> GSVGNREEKILNREIGFAIGMPVCEFDMVKDPEVQDFRRNILNVCKEAVDLRDLNSPHSRAMYVYPPNVESSPELPKHIYNKLDKGQIIVVIWVIVSPNNDKQKYTLKINHDCVPEQVIAEAIRKKTRSMLLSSEQLKLCVLEYQGKYILKVCGCDEYFLEKYPLSQYKYIRSCIMLGRMPNLMLMAKESLYSQLPMDCFTMPSYSRRISTATPYMNGETSTKSLWVINSALRIKILCATYVNVNIRDIDKIYVRTGIYHGGEPLCDNVNTQRVPCSNPRWNEWLNYDIYIPDLPRAARLCLSICSVKGRKGAKEEHCPLAWGNINLFDYTDTLVSGKMALNLWPVPHGLEDLLNPIGVTGSNPNKETPCLELEFDWFSSVVKFPDMSVIEEHANWSVSREAGFSYSHAGLSNRLARDNELRENDKEQLKAISTRDPLSEITEQEKDFLWSHRHYCVTIPEILPKLLLSVKWNSRDEVAQMYCLVKDWPPIKPEQAMELLDCNYPDPMVRGFAVRCLEKYLTDDKLSQYLIQLVQVLKYEQYLDNLLVRFLLKKALTNQRIGHFFFWHLKSEMHNKTVSQRFGLLLESYCRACGMYLKHLNRQVEAMEKLINLTDILKQEKKDETQKVQMKFLVEQMRRPDFMDALQGFLSPLNPAHQLGNLRLEECRIMSSAKRPLWLNWENPDIMSELLFQNNEIIFKNGDDLRQDMLTLQIIRIMENIWQNQGLDLRMLPYGCLSIGDCVGLIEVVRNSHTIMQIQCKGGLKGALQFNSHTLHQWLKDKNKGEIYDAAIDLFTRSCAGYCVATFILGIGDRHNSNIMVKDDGQLFHIDFGHFLDHKKKKFGYKRERVPFVLTQDFLIVISKGAQECTKTREFERFQEMCYKAYLAIRQHANLFINLFSMMLGSGMPELQSFDDIAYIRKTLALDKTEQEALEYFMKQMNDAHH

Class IA PI3Ks signal downstream of tyrosine kinases, G protein-coupled receptors and small GTPases to regulate cell metabolism, growth, proliferation and migration. They consist of a p110α, β or δ catalytic subunit and a p85 regulatory subunit (further referred to as PI3Kα, PI3Kβ and PI3Kδ), with a broad tissue distribution (p110α, p110β) or enriched in leukocytes (p110δ). PI3Kα phosphorylates PIP2 in the plasma membrane to PtdIns(3,4,5)P3 (or PIP3), which can be converted by 5-phosphatases to PtdIns(3,4)P2. Here we report on the discovery of UCL-TRO-1938 (further referred to as 1938), a small molecule activator of the PI3Kα isoform, a critical effector of growth factor signalling.

We next used a deletion variant of p110α (p110α AA105-1048)30 in which the p85 adaptor-binding domain (AA1-104) and a C-terminal membrane binding motif in the kinase domain (AA1049-1068) were deleted. This construct lacks catalytic activity but, in contrast to wild-type p110α, is stable in the absence of p8530. Co-crystallisation with 1938 did not yield crystals, however, soaking preformed crystals with 1938 revealed density for 1938.> RMKGSKEVFLVKFVKSSGSSEYFLKALESIKEFQSEEHLQILEEEAALNIKENDKSLYICDPFTGVVFNH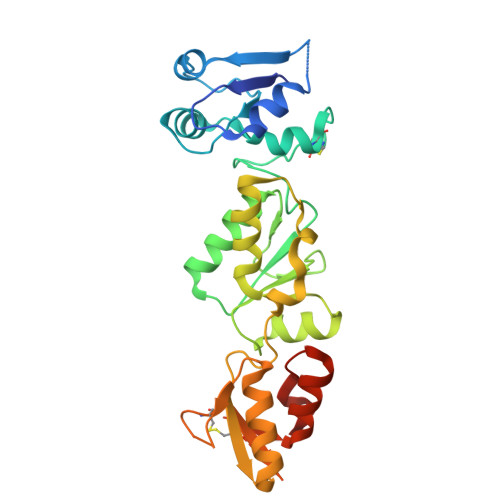LKKLGCRIVGPQVVLYCMQSQRCVPRAEYPVYNMTMADVTISCTTLDKDVREEVHKYVQMMGGRVYRDLNMSVTHLIAGEVGSKKYLVAASLKKPVLLPSWVKTLWDKSQQRMMRYTDVNMEDYACPVFLGCTICVTGLSSSDRKEVQRLTAEHGGQYSGQLKMNECTHLIVQEPKGQKYECAKKWNVHCVPVQWFSDSIEKGFCQDETMYKIESGSKLS>MIHHHHHHEHRHLKPFPPEFLWGAASAAYQVEGAWNEDGKGLSVWDVFAKQPGRTFKGTNGDVAVDHYHRYQEDVALMAEMGLKAYRFSVSWSRVFPDGNGAVNEKGLDFYDRLIEELRNHGIEPIVTLYHWDVPQALMDAYGAWESRRIIDDFDRYAVTLFQRFGDRVKYWVTLNQQNIFISFGYRLGLHPPGVKDMKRMYEANHIANLANAKVIQSFRHYVPDGKIGPSFAYSPMYPYDSRPENVLAFENAEEFQNHWWMDVYAWGMYPQAAWNYLESQGLEPTVAPGDWELLQAAKPDFMGVNYYQTTTVEHNPPDGVGEGVMNTTGKKGTSTSSGIPGLFKTVRNPHVDTTNWDWAIDPVGLRIGLRRIANRYQLPILITENGLGEFDTLEPGDIVNDDYRIDYLRRHVQEIQRAITDGVDVLGYCAWSFTDLLSWLNGYQKRYGFVYVNRDDES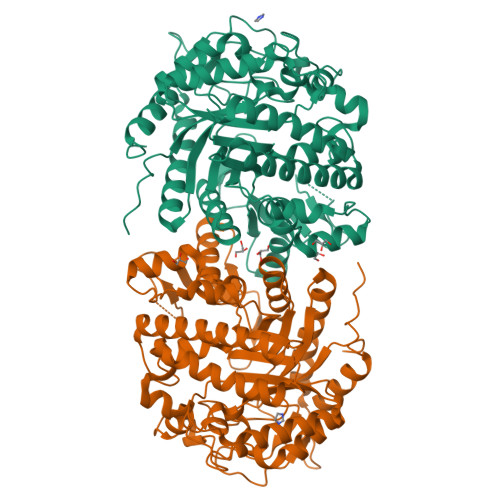EKDLRRIKKKSFYWYQRVIETNGAEL[4x]>MKNENENEICFIAGVGDSNGYGWGIAKELSKRNVKVIFG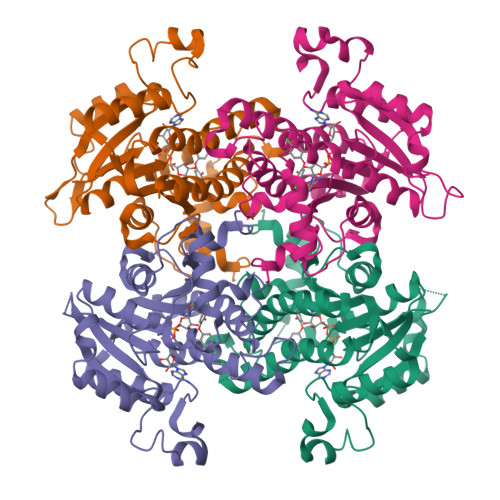VWPPVYNIFIKNLESGKFDKDMIINNDNSKRMQILDVLPLDAGFDNYDDIDEDTKNNKRYNNLKNYSIEEVANLIYNKYGKISMLVHSLANGREVQKSLLDTSRDGYLDAISKSSYSLISLCKHFCKFMNSGGSVVSLTYQASQKVVPGYGGGMSSAKAALESDTRVLAYYLGRKYNIRINTISAGPLKSRAATAINKFNNNQKNNMNSSGETDKQNYSFIDYAIDYSEKYAPLKKKLLSTDVGSVASFLLSKESSAVTGQTIYVDNGLNIMFGPDDLFQSSDS[4x]N,N-dimethyl-1,2,3,4-tetrahydroquinoline-6-carboxamide | C12 H16 N2 O | 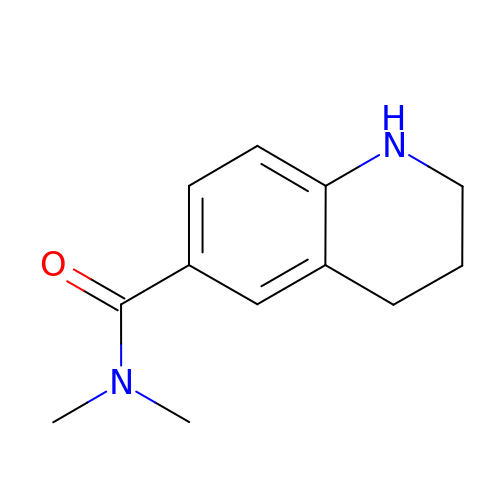WKHXWPZSIXHQAS-UHFFFAOYSA-N>[13x]MASGSNVEEYELDVEALVVILRDRNIPRNPLHGEVIGLRLTEGWWGQIERFQMVRLILQNDDNEPLQRPRYEVIQRAVNPHTMFMISGPLAELQLAFQDLDLPEGPLRFGPLANGHYVQGDPYSSSYRPVTMAETAQMTRDELEDVLNTQSEIEIQMINLLELYEVETRALRRQLAERSSTGQGGISPGAPRSRPPVSSFSGLPSLPSIPGIHPRAPSPPRATSTPGNIPWSLGDDNPPSSSFPGPSQPRVSFHPGNPFVEEEGHRPRSQSRERRREILPAPVPSAPPMIQYIP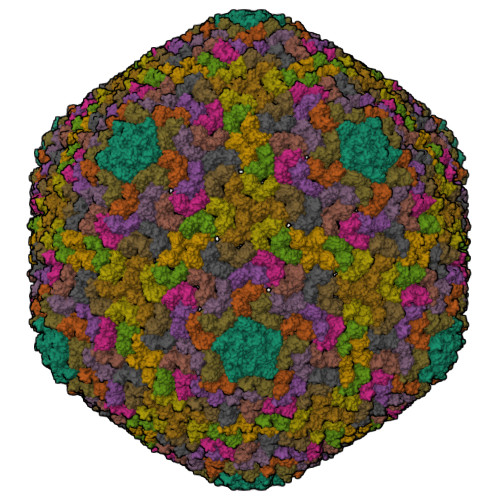VPPPPPIGTVIPIQHIRSVTGEPPRNPREIPIWLGRNAPAIDGVFPVTTPDLRCRIINAILGGNIGLSLTPGDCLTWDSAVATLFIRTHGTFPMHQLGNVIKGIVDQEGVATAYTLGMMLSGQNYQLVSGIIRGYLPGQAVVTALQQRLDQEIDDQTRAETFIQHLNAVYEILGLNARGQSIRASVTPQPRPSRGRGRGQNTSRPSQGPANSGRGRQRPASGQSNRGSSTQNQNQDNLNQGGYNLRPRTYQPQRYGGGRGRRWNDNTNNQESRPSDQGSQTPRPNQAGSGVRGNQSQTPRPAAGRGGRGNHNRNQRSSGAGDSRAVNTVTQSATSSTDESSSAVTAASGGDQRD> MRIGFNFTLGETLPLVRQLAQEGAIDYCELLIDNFMQVPPQELAEAFDVPVGFHIMFSRFIESDEEQLRDFAARLRPYIEALRPLYVSDHIAYFSHQGRALYHLGEIDYAADYERVRARAALWQSLLGQTIHFENYPSIVDGGHAAPAFFQRLARDTGAGV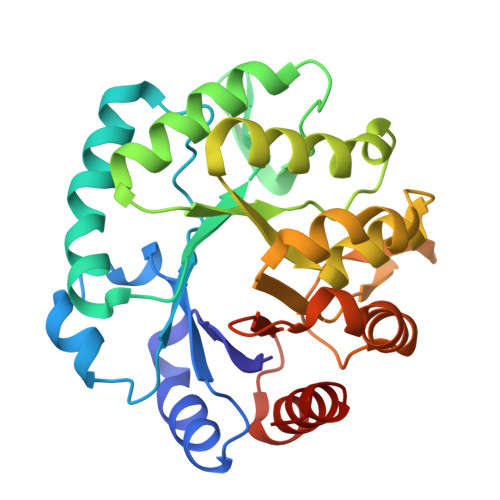LFDVSNAVCAWRNDGPEVAAWRGVMAGASHFHVGGYAGAFIDEGVTVDTHDRALAQDTLDSLRRHRDVLDKPGATITYERDENIDIDGVRADLLALRAIFPR> GLPVLNTPGSNQYLTADNYQSPCAIPEFDVTPPIDIPGEVRNMMELAEIDTMIPLNLTNQRKNTMDMYRVELNDAAHSDTPILCFSLSPASDPRLAHTMLGEILNYYTHWAGSLKFTFLFCGSMMATGKLLVSYAPPGAEAPKSRKEAMLGT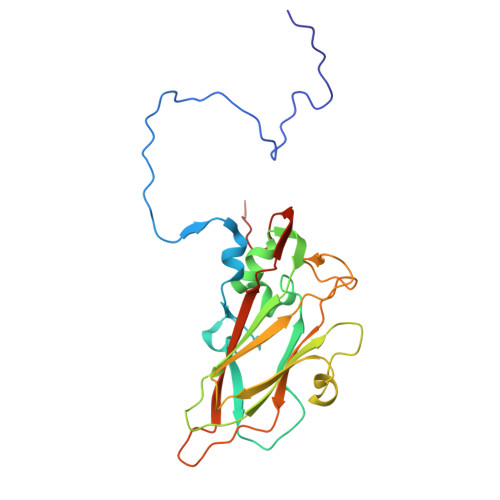HVIWDIGLQSSCTMVVPWISNTTYRLTINDSFTEGGYISMFYQTRVVVPLSTPRKMDILGFVSACNDFSVRLLRDTTHISQEAMPQ> GSHMRKQEELTDEEK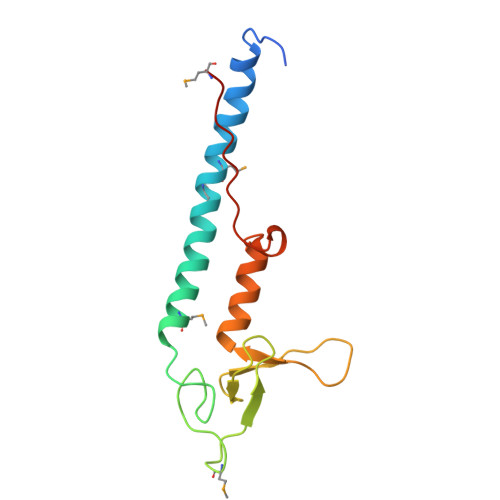EIINRVIARAEKMETMEQERIGRLVDRLETMRKNVAGDGVNRCILCGEQLGMLGSASVVCEDCKKNVCTKCGVETSNNRPHPVWLCKICLEQREVWKRSGAWFFKGFPKQVLPQPMPIK>[2x]MVKNWLFGKKRKEDADALATLKGQQNRLQAEARNLERQSDEQKILASKMLKAGNKAGARQALKRRAVFMKRLNTVHNTAMNLQAQIDSIQTATSTAETVKAMELGTK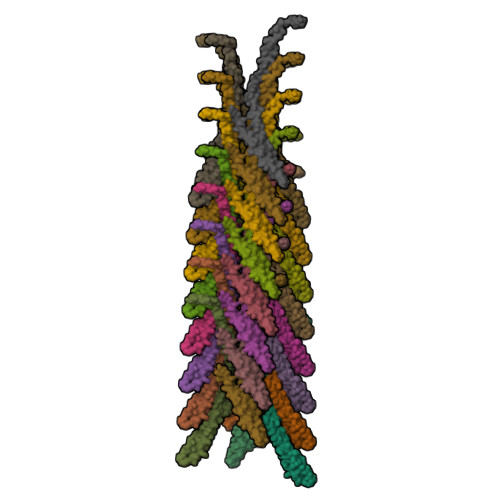VVGEKIKTVSPERTERVMDSVMEQRDQIEMMTEALSDPSLSEGILDFEDDAAIDEQLAQLEAEMDLGTTTSLPDVSGLPSTPVGTGEKEEDTSELEAELEGLKKKMSEDKQ> MGSSHHHHHHSQGSMTDDKDVLRDVWFGRIPTCFTLYQDEITEREAEPYYLLLPRVSYLTLVTDKVKKHFQKVMRQEDISEIWFEYEGTPLKWHYPIGLLFD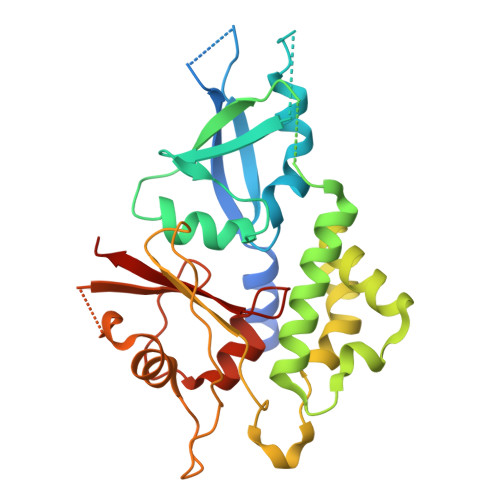LLASSSALPWNITVHFKSFPEKDLLHCPSKDAIEAHFMSCMKEADALKHKSQVINEMQKKDHKQLWMGLQNDRFDQFWAINRKLMEYPAEENGFRYIPFRIYQTTTERPFIQKLFRPVAADGQLHTLGDLLKEVCPSAIDPEDGEKKNQVMIHGIEPMLETPLQWLSEHLSYPDNFLHISIIPQPTD>MWSHPQFEKGSGSENLYFQGGGGGKVINDPIHGHIELHPLLVRIIDTPQFQRLRYIKQLGGGYYVFPGASHNRFEHSLGVGYLAGCLVHALGEKQPELQISERDVLCVQIAGLCHDLGHGPFSHMFDGRFIPLARPEVKWTHEQGSVMMFEHLINSNGIKPVMEQYGLIPEEDICFIKEQIVGPLESPVEDSLWPYKGRPENKSFLYEIVSNKRNGIDVDKWDYFARDCHHLGIQNNFDYKRFIKFARVCEVDNELRICARDKEVGNLYDMFHTRNSLHRRAYQHKVGNIIDTMITDAFLKADDYIEITGAGGKKYRISTAIDDMEAYTKLT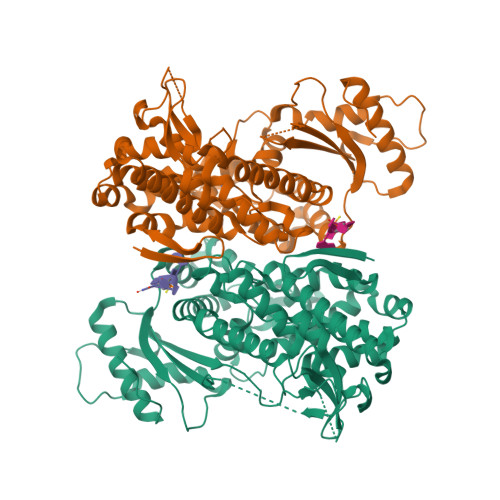DNIFLEILYSTDPKLKDAREILKQIEYRNLFKYVGETQPTGQIKIKREDYESLPKEVASAKPKVLLDVKLKAEDFIVDVINMDYGMQEKNPIDHVSFYCKTAPNRAIRITKNQVSQLLPEKFAEQLIRVYCKKVDRKSLYAARQYFVQWCADRNFTKPQDGDVIAPLITPQKKEWNDSTSVQNPTRLREASKSRVQLFKDDPM[4x]The HNV F protein is a trimeric type I fusion protein that is initially expressed as an F precursor (F0), consisting of three domains (DI, DII and DIII), a C-terminal stem, a transmembrane domain and a cytoplasmic tail. We found that LayV F and MojV F both adopt a “tree-like” prefusion F structure similar to that of NiV, despite only sharing ~40% sequence conservation at the amino acid level. We show that despite sequence divergence from NiV, the F proteins adopt an overall similar structure but are antigenically distinct as they do not react to known antibodies or sera.

Indeed, 2D class averages generated from initial cryo-EM images revealed particles resembling the canonical three-fold symmetry HNV F protein structure. Concurrently, we applied the same methodology to MojV F, where ectodomain residues 1–482 were used to express the prefusion conformation. Next, we determined the structure of MojV F to 2.66 Å. Here, a total of ~260,000 particles were extracted and 2D classified from ~9000 curated movies. These were further classified using ab initio and heterogenous refinements within cryoSPARC to yield ~214,000 particles that were subsequently used in a homogenous refinement. Interestingly, while the stem domain for MojV was observed in 2D classes, this region was not observed in any 3D classification or homogenous refinements and therefore was not resolved to a high resolution. Structural comparisons of LayV and MojV F ectodomains revealed several surface exposed, conserved (L23I, I33V, R64K, F71Y, K79R, L89I, K197R, L206I, E267D, V298I, V328I, E330D, Y345H, R370K, K411R, I420V, E430D, V444I) and non-conserved (G62S, N80K, V81A, L87M, N90D, A91T, D94N, N144S, R232G, G255E, T402A, L413S, S434N, N468E) substitutions in DI, DII and DIII. These are differences that should be noted, however we anticipate that cross-reactive responses between the two would be possible, given the high sequence similarity in the F glycoproteins (~90%). Despite an overall high structural resemblance between NiV prefusion F and the divergent LayV (RMSD = 1.8 Å) and MojV F (RMSD = 2.6 Å) structures, there are some notable differences. Comparison of the trimers reveals a shift in the major outward facing DIII helix of LayV F relative to NiV, mediated by an adjacent loop region of a neighbouring protomer, which adopts an altered conformation in both MojV and LayV. Conversely, the F1/F2 cleavage site of LayV more closely resembles the NiV and HeV site, despite high sequence homology between LayV and MojV in this region.

>MALNKNMFSSLFLGYLLVYATTVQSSIHYDSLSKVGVIKGLTYNYKIKGSPSTKLMVVKLIPNIDSVKNCTQKQYDEYKNLVRKALEPVKMAIDTMLNNVKSGNNKYRFAGAIMAGVALGVATAATVTAGIALHRSNENAQAIANMKSAIQNTNEAVKQLQLANKQTLAVIDTIRGEINNNIIPVINQLSCDTIGLSVGIRLTQYYSEIITAFGPALQNPVNTRITIQAISSVFNGNFDELLKIMGYTSGDLYEILHSELIRGNIIDVDVDAGYIALEIEFPNLTLVPNAVVQELMPISYNIDGDEWVTLVPRFVLTRTTLLSNIDTSRCTITDSSVICDNDYALPMSHELIGCLQGDTSKCAREKVVSSYVPKFALSDGLVYANCLNTICRCMDTDTPISQSLGATVSLLDNKRCSVYQVGDVLISVGSYLGDGEYNADNVELGPPIVIDKIDIGNQLAGINQTLQEAEDYIEKSEEFLKG[3x]>[2x]GHSGKPIPNPLLGLDSTHMFPRFRELYYITHIDNVPSILEKGILSHAEIERQSINCKKVYDNSIVLKRKSRLLADNRSLWEFANLYFQPRNPMLYRLLVQGLKPKDLAIVAVKWTIMKRDDILITDGNAASSETQIYRKSEIKNIKNIISVKDMEYWREEDGSKRKIMAACLVPQCVDPRYISAIYVSDHEVASNLKKAINNRNIPVIPDPTFFFLPNREIKLTQNLSLVEGDMFFSRMQTL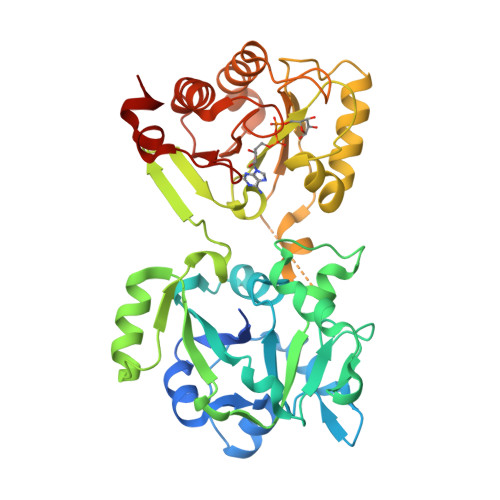TVSVNTVGVMGKGLASRVKYQFPDVYVVFQDACKKKELEFGKPYLYKRESSLDAFLAEDGEKLSDLNHQTWFLLFPTKRHWKNMSEIKGIESGLRWIVENYKKEGIKSLAVPALGCGLGGLEWSIVGPLMCRYLTKLEIPVQIYLPLEKRIPDVQLSPKFLLDS>[2x]SHMAHQDALPRLPVPPLQQSLDYYLKALQPIVSEEEWAHTKQLVDEFQTSGGVGERLQKGLERRAKKMENWLSEWWLKTAYLQFRQPVVIYSSPGVILPKQDFVDLQGQLRFAAKLIEGVLDFKSMIDNETLPVEFLGGQPLCMNQYYQILSSCRVPGPKQDSVVNFLKSKRPPTHITVVHNYQFFELDVYHSDGTPLTSDQIFVQLEKIWNSSLQSNKEPVGILTSNHRNTWAKAYNNLIKDKVNRESVNSIQKSIFTVCLDKQVPRVSDDVYRNHVAGQMLHGGGSKFNSGNRWFDKTLQFIVAEDGSCGMVYEHAAAEGPPIVALVDHVMEYTKKPELVRSPMVPLPMPKKLRFNITPEIKNDIEKAKQNLSIMIQDLDIMMLTFHHFGKDFPKSEKLSPDAFIQVALQLAYYR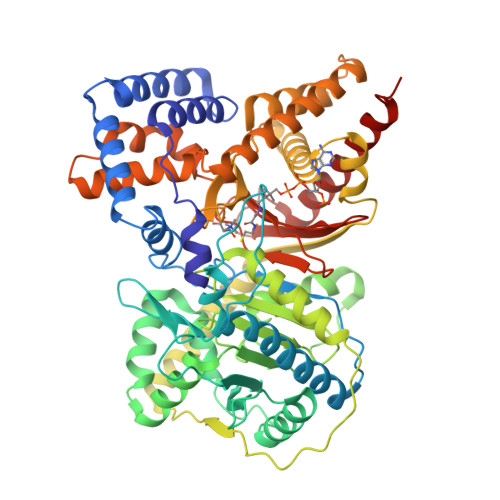IYGQACATYESASLRMFHLGRTDTIRSASIDSLAFVKGMGDSTVPEQQKVELLRKAVQAHRAYTDRAIRGEAFDRHLLGLKLQAIEDLVSMPDIFMDTSYAIAMHFNLSTSQVPAKTDCVMFFGPVVPDGYGICYNPMEAHINFSVSAYNSCAETNAARMAHYLEKALLDMRTLLQNHPRAK> DAILDEIDDVLEENAEEFVRSYIQKG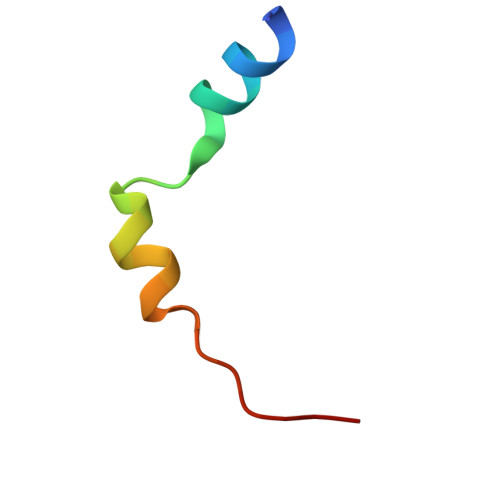GQ>[2x]MAHHHHHHVDDDDKTFKMNTAQKAHYEKFINALENELKTRHIPAGAVIDMLAEINTE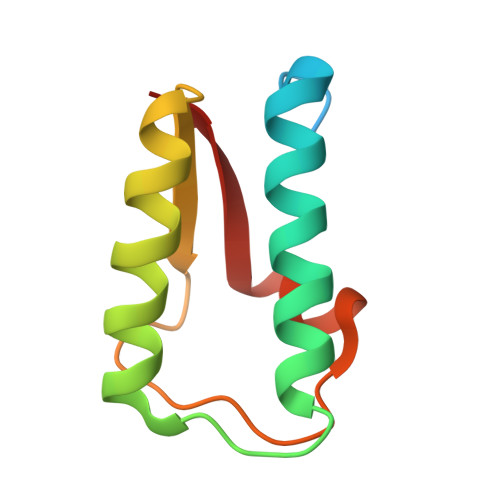ALALDYQIVDKKPGTSIAQGTKAAALRKRFIPKKIK>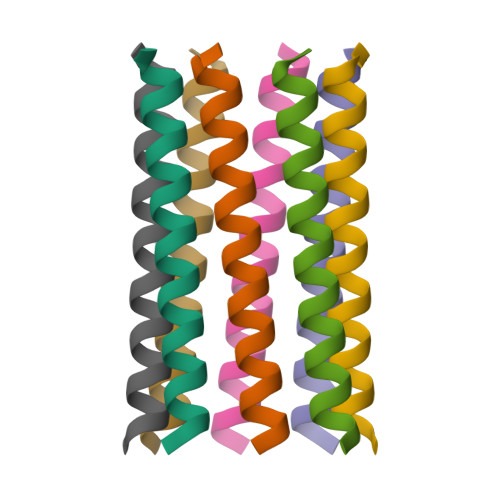[2x]XGEIAQALKEIAKALKEIAWALKENAQALKGX>GCGGGGACGACCCCGC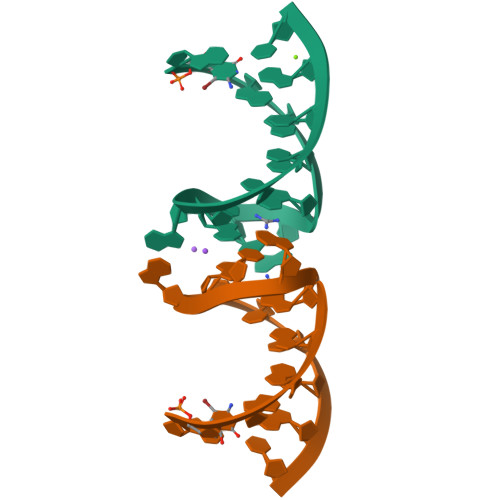[4x]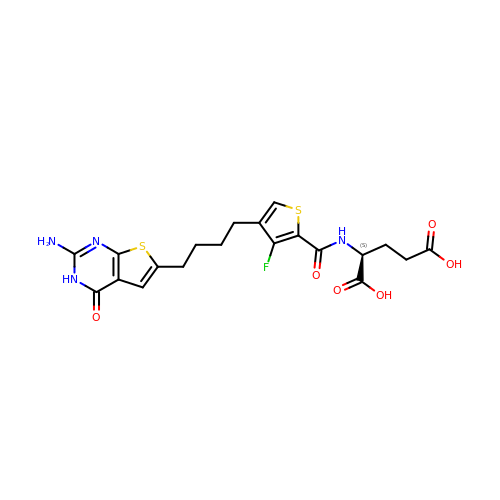N-{4-[4-(2-amino-4-oxo-3,4-dihydrothieno[2,3-d]pyrimidin-6-yl)butyl]-3-fluorothiophene-2-carbonyl}-L-glutamic acid | C20 H21 F N4 O6 S2 | WMUHYWZCFKANFD-LBPRGKRZSA-N> MRAPIPEPKPGDLIEIFRPFYRHWAIYVGDGYVVHLAPPSEVAGAGAASVMSALTDKAIVKKELLYDVAGSDKYQVNNKHDDKYSPLPCSKIIQRAEELVGQEVLYKLTSENCEHFV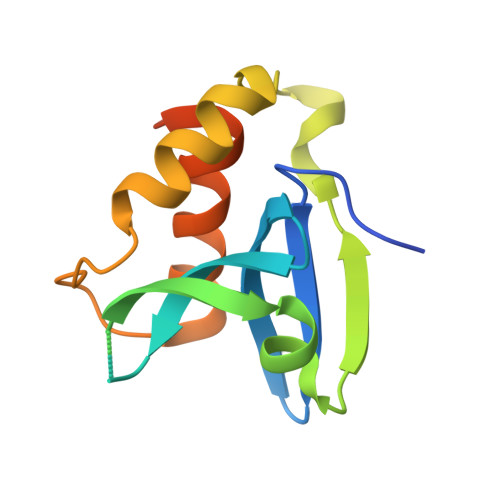NELRYGVARSDQVRDLEHHHHHH> GSHMSNISLIVGLGNPGSEYAQTRHNAGFWFVEQLADKYGITLKNDPKFHGISGRGNIEGHDVRLLLPMTYMNRSGQSVVPFSKFYQIAPEAILIAHDELDMNPGVIRLKTGGGHGGHNGLRDIVPHIGPNFHRLRIGIGHPGSKERVSGHVLGKAPSNEQSLMDGAIDHALSKVKLLV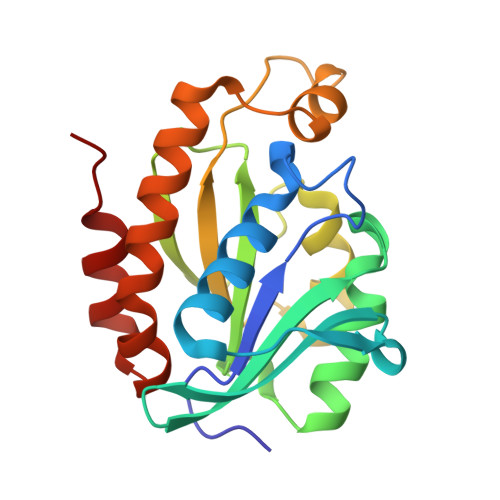QGQVPQAMNQINAYKPA>MANLTEKFLRIFARRGKSIILAYDHGIEHGPADFMDNPDSADPEYILRLARDAGFDGVVFQRGIAEKYYDGSVPLILKLNGKTTLYNGEPV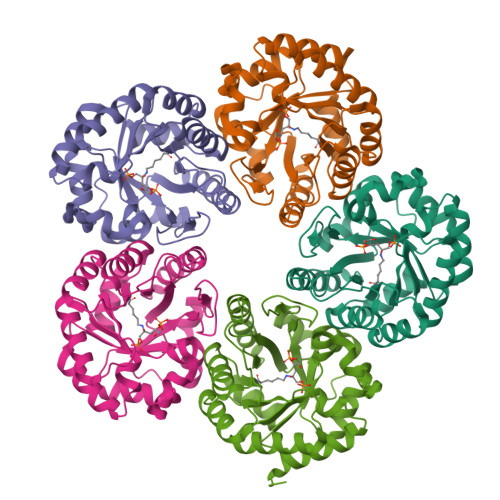SVANCSVEEAVSLGASAVGYTIYPGSGFEWKMFEELARIKRDAVKFDLPLVVWSFPRGGKVVNETAPEIVAYAARIALELGSDAMKIKYTGDPKTFSWAVKVAGKVPVLMSGGPKTKTEEDFLKQVEGVLEAGALGIAVGRNVWQRRDALKFARALAELVYGGKKLAEPLNV[10x]> MCEPVS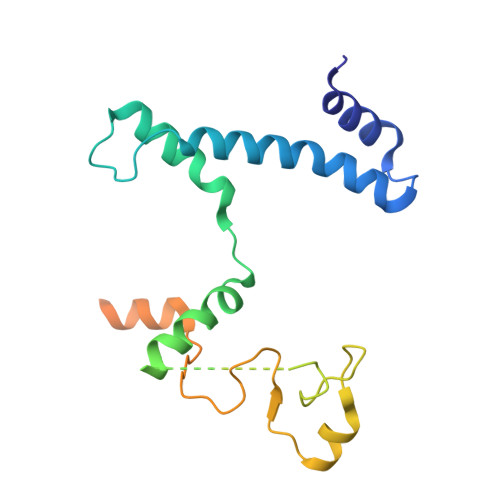IGLGIMSVAGATMSASQQAKAEGAAIDAQNRQAQEMIKQMNYSDANLKMQERDLKEQQMAELTETTLNGIRNQGMVRAAVAESGLEGNSMDRIERQVAGDTVKERAGITESYNRDYAAIFGNRIANIENTQSAIRGQGKIIKTSPLAHALNVATAGVQGYAAGKSMSGTSGSGGAAPISAAKGTPTGHS>MESEQLFHRGYYRNSYNSITSASSDEELLDGAGVIMDFQTSEDDNLLDGDTAVGTHYTMTNGGSINSSTHLLDLLDEPIPGVGTYDDFHTIDWVREKCKDRERHRRINSKKKESAWEMTKSLYDAWSGWLVVTLTGLASGALAGLIDIAADWMTDLKEGICLSALWYNHEQCCWGSNETTFEERDKCPQWKTWAELIIGQAEGPGSYIMNYIMYIFWALSFAFLAVSLVKVFAPYACGSGIPEIKTILSGFIIRGYLGKWTLMIKTITLVLAVASGLSLGKEGPLVHVACCCGNIFSYLFPKYSTNEAKKREVLSAASAAGVSVAFGAPIGGVLFSLEEVSYYFPLKTLWRSFFAALVAAFVLRSINPFGNSRLVLFYVEYHTPWYLFELFPFILLGVFGGLWGAFFIRANIAWCRRRKSTKFGKYPVLEVIIVAAITAVIAFPNPYTRLNTSELIKELFTDCGPLESSSLCDYRNDMNASKIVDDIPDRPAGIGVYSAIWQLCLALIFKIIMTVFTFGIKVPSGLFIPSMAIGAIAGRIVGIAVEQLAYYHHDWFIFKEWCEVGADCITPGLYAMVGAAACLGGVTRMTVSLVVIVFELTGGLEYIVPLMAAVMTSKWVGDAFGREGIYEAHIRLNGYPFLDAKEEFTHTTLAADVMRPRRNDPPLAVLTQDNMTVDDIENMINETSYNGFPVIMSKESQRLVGFALRRDLTIAIESARKKQEGIVGSSRVCFAQHTPSLPAESPRPLKLRSILDMSPFTVTDHTPMEIVVDIFRKLGLRQCLVTHNGRLLGIITKKDILRHMAQTANQDPASIMFN[2x];>MKLLSLVAVVGCLLVPPAEANKSSEDIRCKCICPPYRNISGHIYNQNVSQKDCNCLHVVEPMPVPGHDVEAYCLLCECRYEERSTTTIKVIIVIYLSVVGALLLYMAFLMLVDPLIRKPDAYTEQLHNEEENEDARSMAAAAASLGGPRANTVLERVEGAQQRWKLQVQEQRKTVFDRHKMLS[2x]

Five members of the CLC family of Cl− channels and Cl−/H+ exchangers, ClC-3, ClC-4, ClC-5, ClC-6 and ClC-7, have critical roles in endosomes and lysosomes, catalyzing the exchange of two Cl− ions for one H+ ion2,10–12. We recently found that the ClC-3, ClC-4 and ClC-5 clade of endosomal CLC transporters requires the accessory β-subunit TMEM9, which we refer to as T9A or its closely related homolog TMEM9B (T9B) for proper activity in cells and animals. To resolve the mechanism by which T9A and T9B regulate the activity of ClC-3, ClC-4 and ClC-5, we determined structures of ClC-3 alone and in complex with T9A, finding that T9A occludes the Cl− ion pathway and that inhibition requires the endolysosomal signaling lipid phosphatidylinositol 3,5-bisphosphate (PtdIns(3,5)P2). Each ClC-3 protomer comprises a cytosolic N-terminal domain (NTD), a transmembrane domain (TMD) and a cytosolic domain (CD).

Analysis of cryo-EM images of ClC-3 in complex with T9A revealed four classes that can be distinguished by the densities corresponding to T9A. We also identified two asymmetric classes in which the densities corresponding to the T9A protomers were incompletely resolved, with the LD and/or CD of T9A being partially or completely disordered. The weak density for these domains suggests that they are more dynamic than the TMD. In addition to ClC-3/T9A, we observed two classes of the complex in which one or both T9A CDs are disordered. The TMDs are resolved in these classes, indicating that the disordered CDs are present but not bound to ClC-3, which is consistent with immunoprecipitation analysis that demonstrated that the LD and the TMD but not the CD are required for the interaction between ClC-3 and T9A29. The disengagement of the T9A CD exposes the cytosolic entrance to the Cl− ion pathway, indicating that these correspond to disinhibited states. We, therefore, propose that the T9A CD blocks access to the Cl− ion pathway through a ball-and-chain-like mechanism. Densities corresponding to PtdIns(3,5)P2 are also resolved in the asymmetric ClC-3/T9A reconstructions.> HMMENINIVIKDVGYFQDKPQFLNSKSVR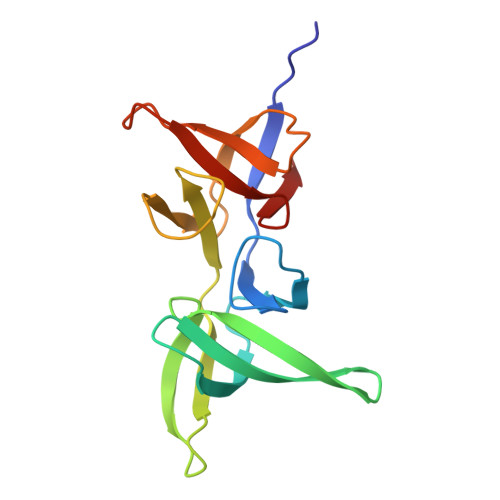QWKHGTKVKLTKHNSHWYTGVVKDGNKSVRGYIYHSMAKVTSKNSDGSVNATINAHAFCWDNKKLNGGDFINLKRGFKGITHPASDGFYPLYFASRKKTFYIPRYMFDIKK>MISGLSHITLI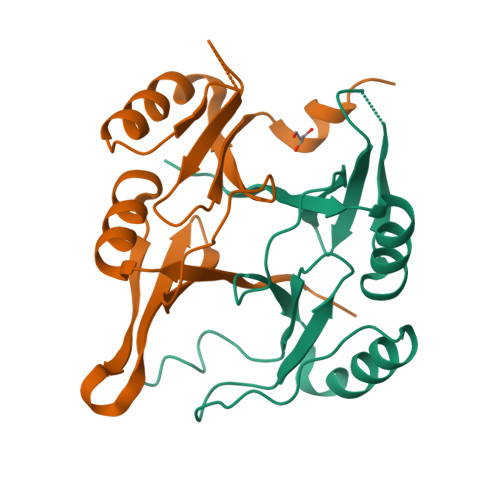VKDLNKTTAFLQNIFNAEEIYSSGDKTFSLSKEKFFLIAGLWICIMEGDSLQERTYNHIAFQIQSEEVDEYTERIKALGVEMKPERPRVQGEGRSIYFYDFDNHLFELHAGTLEERLKRYHE[6x]>MVRRRGGKTAGSKRPKMSSKNFGANRKRDFRRPARKSKAKKARSMAPAKTVRKSTTAGAHSKHFSVIGNPFSKATQQPQIPDGRMLESLPRRCQLVTEIRNNVTVGSNPTYILVAPSLGLAFQAYQDTNVPGGLDSSVYGLQNRGCTVRANLSATSIENYNDIAKWRIVSQGINLKLNNVEDENDGWYEACRFQHDWTPDELCLRSTENDASTISQDEDLVMGVISSSFMNGALNTIGNNMVEQRGYESGLLKNIHKRMFQLHNNTSAIRPKTLQGQFNYGSEITFSGTESEARFTDVPSNRQLVDSLWHNDYDCILIKLYPRENTGAAGQTGSALIVNAIQNLELQYSPTSDLSTYHIANKRARMVEAKLDKKNNTDAAGEPFVPGSSR[3x]

Bacilladnaviruses is one of the major group of viruses infecting eukaryotic algae. They carry a circular ssDNA genome of ~6 kb, which is partially double stranded (~700 to 800 bp) and encodes three proteins; one coat protein, one replication-associated protein (Rep), and a third protein with unknown function. We present the capsid structure of the bacilladnavirus Chaetoceros tenuissimus DNA virus type II (CtenDNAV-II), determined at 2.4-Å resolution. The capsid protein contains the widespread virus jelly-roll fold but has additional unique features; a third β-sheet and a long C-terminal tail.

The capsid was reconstructed by imposing icosahedral symmetry (I4) and using 33,507 particles to an overall resolution of 2.4 Å using the “gold standard” Fourier shell correlation (FSC) 0.143 criterion. The CtenDNAV-II capsid displays T = 3 symmetry, i.e., 180 capsid protein protomers assemble such that the asymmetric unit comprises 3 capsid subunits in 3 quasiequivalent positions termed A, B, and C. For subunit A and B, residues 64 to 371 were modeled, and for subunit C, residues 60 to 365 and 378 tp 384 were modeled. The A and B subunits were close to identical: the C terminus of the A and B subunits form long tails that end on the capsid surface around the 3- and 5-fold axes, respectively. Contrary to the long tail toward the capsid surface, the C terminus of the C subunit is directed toward the capsid interior. The N terminus of the C subunit has a small α-helix on the capsid interior that was not present in the other two subunits. For CtenDNAV-II, the two sheets are formed by strands BIDD’G and C″C’CHEF, respectively, thus containing three additional strands (D’, C,’ and C″) compared to the standard viral jelly-roll fold. In addition, a third antiparallel β-sheet with seven strands is intertwined within the jelly-roll, i.e., strands from the third sheet are formed by extensions of loops CD, EF, and GH of the jelly-roll. The unmodeled density in the subunit interface of CtenDNAV-II has a pyramidal to spherical shape and is surrounded by six arginine residues (R84 and R270) that resemble an octahedral coordination geometry. CtenDNAV-II is placed together with RNA viruses from families Nodaviridae, Alphatetraviridae, Carmotetraviridae, and Birnaviridae (Clade 1), thus corroborating the result from the DALI search as well as the previous HGT theory by Kazlauskas et al..> MDDEDNKCDCPPPGLPLW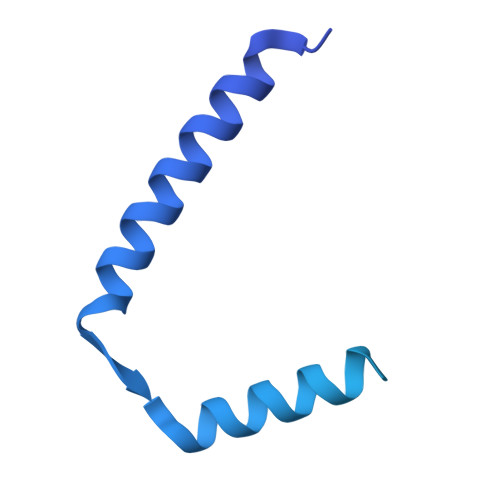MGTFANLMSLLMCFFVLLLSFSEMDVLKFKQIAGSMKFAFGVQNQLEVKDIPKGTSIIAQEFRPGRPEPTPIDVIMQQTMDITQQTLEFHEGESDRAGGTKRDEGKLTGGQSPATSTQNNESAEADMQQQQSKEMSQEMETLMESIKKALEREIEQGAIEVENLGQQIVIRMREKGAFPEGSAFLQPKFRPLVRQIAELVKDVPGIVRVSGHTDNRPLDSELYRSNWDLSSQRAVSVAQEMEKVRGFSHQRLRVRGMADTEPLLPNDSDDNRALNRRVEISIMQGEPLYSEEVPVIQHHHHHH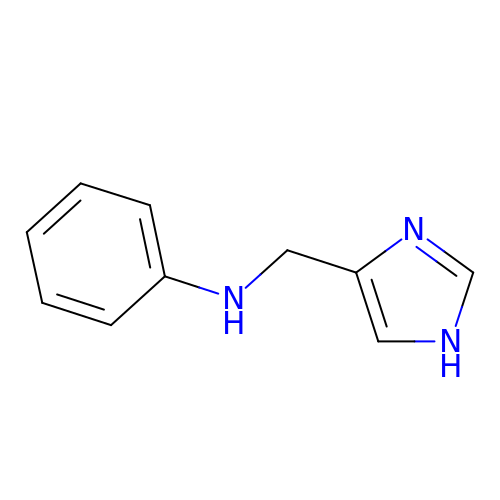N-[(1H-imidazol-4-yl)methyl]aniline | C10 H11 N3 | AUZUSOIPPYQZQA-UHFFFAOYSA-N The gamma-tubulin ring complex (γ-TuRC) is the principal microtubule nucleation template in vertebrates. Microtubules are formed de novo in a process termed nucleation, which is spatially and temporally highly controlled by γ-tubulin complexes, composed of γ-tubulin1 and associated γ-tubulin-complex proteins (GCP). In most eukaryotes, microtubules are templated from a preassembled γ-tubulin ring complex (γ-TuRC) that determines the position and direction of microtubule growth. Here, we used cryo-EM to identify and characterize γ-TuRC assembly intermediates after recombinant expression of the complex, which allowed us to delineate a comprehensive stepwise assembly pathway from a stable 6-spoked core to the mature 14-spoked γ-TuRC, identifying successive stabilization and conformational locking of γ-TuSC units as central principles in the assembly process.

The almost constant ratio between γ-TuSC(13,14)-containing and -lacking intermediates for each assembly step argues for repeated association and dissociation of γ-TuSC(13,14) in an equilibrium reaction. Stable incorporation of the γ-TuSC(13,14) unit, which is likely to repeatedly associate and dissociate over the assembly process, is a two-step process. Collectively, the observed intermediate steps can be arranged into a pathway for modular assembly of the γ-TuRC, in which the 6-spoke intermediate is expanded by successive recruitment of γ-TuSC units on the GCP2(7)-facing side while the γ-TuSC(13,14) unit repeatedly associates and dissociates until it is stabilized in the final step of complex assembly.

>[8x]MPREIITLQLGQCGNQIGFEFWKQLCAEHGISPEGIVEEFATEGTDRKDVFFYQADDEHYIPRAVLLDLEPRVIHSILNSPYAKLYNPENIYLSEHGGGAGNNWASGFSQGEKIHEDIFDIIDREADGSDSLEGFVLCHSIAGGTGSGLGSYLLERLNDRYPKKLVQTYSVFPNQDEMSDVVVQPYNSLLTLKRLTQNADCVVVLDNTALNRIATDRLHIQNPSFSQINQLVSTIMSASTTTLRYPGYMNNDLIGLIASLIPTPRLHFLMTGYTPLTTDQSVASVRKTTVLDVMRRLLQPKNVMVSTGRDRQTNHCYIAILNIIQGEVDPTQVHKSLQRIRERKLANFIPWGPASIQVALSRKSPYLPSAHRVSGLMMANHTSISSLFERTCRQYDKLRKREAFLEQFRKEDMFKDNFDEMDTSREIVQQLIDEYHAATRPDYISWGTQEQ;>MSEFRIHHDVNELLSLLRVHGGDGAEVYIDLLQKNRTPYVTTTVSAHSAKVKIAEFSRTPEDFLKKYDELKSKNTRNLDPLVYLLSKLTEDKETLQYLQQNAKERAELAAAAVGSSTTSINVPAAASKISMQELEELRKQLGSVATGSTLQQSLELKRKMLRDKQNKKNSGQHLPIFPAWVYERPALIGDFLIGAGISTDTALPIGTLPLASQESAVVEDLLYVLVGVDGRYVSAQPLAGRQSRTFLVDPNLDLSIRELVHRILPVAASYSAVTRFIEEKSSFEYGQVNHALAAAMRTLVKEHLILVSQLEQLHRQGLLSLQKLWFYIQPAMRTMDILASLATSVDKGECLGGSTLSLLHDRSFSYTGDSQAQELCLYLTKAASAPYFEVLEKWIYRGIIHDPYSEFMVEEHELRKERIQEDYNDKYWDQRYTIVQQQIPSFLQKMADKILSTGKYLNVVRECGHDVTCPVAKEIIYTLKERAYVEQIEKAFNYASKVLLDFLMEEKELVAHLRSIKRYFLMDQGDFFVHFMDLAEEELRKPVEDITPPRLEALLELALRMSTANTDPFKDDLKIDLMPHDLITQLLRVLAIETKQEKAMAHADPTELALSGLEAFSFDYIVKWPLSLIINRKALTRYQMLFRHMFYCKHVERQLCSVWISNKTAKQHSLHSAQWFAGAFTLRQRMLNFVQNIQYYMMFEVMEPTWHILEKNLKSASNIDDVLGHHTGFLDTCLKDCMLTNPELLKVFSKLMSVCVMFTNCMQKFTQSMKLDGELGGQTLEHSTVLGLPAGAEERARKELARKHLAEHADTVQLVSGFEATINKFDKNFSAHLLDLLARLSIYSTSDCEHGMASVISRLDFNGFYTERLERLSAERSQKATPQVPVLRGPPAPAPRVAVTAQ[2x];>MATPDQKSPNVLLQNLCCRILGRSEADVAQQFQYAVRVIGSNFAPTVERDEFLVAEKIKKELIRQRREADAALFSELHRKLHSQGVLKNKWSILYLLLSLSEDPRRQPSKVSSYATLFAQALPRDAHSTPYYYARPQTLPLSYQDRSAQSAQSSGSVGSSGISSIGLCALSGPAPAPQSLLPGQSNQAPGVGDCLRQQLGSRLAWTLTANQPSSQATTSKGVPSAVSRNMTRSRREGDTGGTMEITEAALVRDILYVFQGIDGKNIKMNNTENCYKVEGKANLSRSLRDTAVRLSELGWLHNKIRRYTDQRSLDRSFGLVGQSFCAALHQELREYYRLLSVLHSQLQLEDDQGVNLGLESSLTLRRLLVWTYDPKIRLKTLAALVDHCQGRKGGELASAVHAYTKTGDPYMRSLVQHILSLVSHPVLSFLYRWIYDGELEDTYHEFFVASDPTVKTDRLWHDKYTLRKSMIPSFMTMDQSRKVLLIGKSINFLHQVCHDQTPTTKMIAVTKSAESPQDAADLFTDLENAFQGKIDAAYFETSKYLLDVLNKKYSLLDHMQAMRRYLLLGQGDFIRHLMDLLKPELVRPATTLYQHNLTGILETAVRATNAQFDSPEILRRLDVRLLEVSPGDTGWDVFSLDYHVDGPIATVFTRECMSHYLRVFNFLWRAKRMEYILTDIRKGHMCNAKLLRNMPEFSGVLHQCHILASEMVHFIHQMQYYITFEVLECSWDELWNKVQQAQDLDHIIAAHEVFLDTIISRCLLDSDSRALLNQLRAVFDQIIELQNAQDAIYRAALEELQRRLQFEEKKKQREIEGQWGVTAAEEEEENKRIGEFKESIPKMCSQLRILTHFYQGIVQQFLVLLTTSSDESLRFLSFRLDFNEHYKAREPRLRVSLGTRGRRSSHT[4x];>MIHELLLALSGYPGSIFTWNKRSGLQVSQDFPFLHPSETSVLNRLCRLGTDYIRFTEFIEQYTGHVQQQDHHPSQQGQGGLHGIYLRAFCTGLDSVLQPYRQALLDLEQEFLGDPHLSISHVNYFLDQFQLLFPSVMVVVEQIKSQKIHGCQILETVYKHSCGGLPPVRSALEKILAVCHGVMYKQLSAWMLHGLLLDQHEEFFIKQGPSSGNVSAQPEEDEEDLGIGGLTGKQLRELQDLRLIEEENMLAPSLKQFSLRVEILPSYIPVRVAEKILFVGESVQMFENQNVNLTRKGSILKNQEDTFAAELHRLKQQPLFSLVDFEQVVDRIRSTVAEHLWKLMVEESDLLGQLKIIKDFYLLGRGELFQAFIDTAQHMLKTPPTAVTEHDVNVAFQQSAHKVLLDDDNLLPLLHLTIEYHGKEHKADATQAREGPSRETSPREAPASGWAALGLSYKVQWPLHILFTPAVLEKYNVVFKYLLSVRRVQAELQHCWALQMQRKHLKSNQTDAIKWRLRNHMAFLVDNLQYYLQVDVLESQFSQLLHQINSTRDFESIRLAHDHFLSNLLAQSFILLKPVFHCLNEILDLCHSFCSLVSQNLGPLDERGAAQLSILVKGFSRQSSLLFKILSSVRNHQINSDLAQLLLRLDYNKYYTQAGGTLGSFGM[2x];>[2x]MARHGPPWSRLDAQQERDVRELVRGVAGLQDEADPNFQLALNFAWSNFRFHRFLDVNSHKIEKTIEGIYEKFVIHSDLSKAASWKRLTEEFLNAPLPSIKEIKTDAHYSILSLLLCLSDSPSNSSYVETPRNKEVEKKDDFDWGKYLMEDEEMDIGPYMDTPNWSEESEEENDQQPLSREDSGIQVDRTPLEEQDQNRKLDPCISWKDEPDDRSWLEHHVVHQYWTARPSQFPHSLHLHSNLAAVWDQHLYSSDPLYVPDDRVLVTETQVIRETLWLLSGVKKLFIFQLIDGKVTVRNNIIVTHLTHSCLRSVLEQIAAYGQVVFRLQEFIDEVMGHSSESMLPGSGSVPKKSTEAPFRTYQAFMWALYKYFISFKEELAEIEKCIINNDTTITLAIVVDKLAPRLSQLKVLHKVFSTGVAEVPPDTRNVVRASHLLNTLYKAILEYDNVGEASEQTVSLLFSLWVETVRPYLQTVDEWIVHGHLWDGAREFIIQRNKNVPVNHRDFWYATYTLYSVSEKTENEEKMSDNASASSGSDQGPSSRQHTMVSFLKPVLKQIIMAGKSMQLLKNLQCAESTTCQAGARDAERKSLYTLFLESVQSRLRHGEDSTPQVLTEQQATKENLMKMQSIAESHLELDDVHDPLLAINFARMYLEQSDFHEKFAGGDVCVDRSSESVTCQTFELTLRSCLYPHIDKQYLDCCGNLMQTLKKDYRLVEYLQAMRNFFLMEGGDTMYDFYTSIFDKIREKETWQNVSFLNVQLQEAVGQRYPEDSSRLSISFENVDTAKKKLPVHILDGLTLSYKVPWPVDIVISLECQKIYNQVFLLLLQIKWAKYSLDVLLFGELVSTAEKPRLKEGLIHEQDTVAQFGPQKEPVRQQIHRMFLLRVKLMHFVNSLHNYIMTRILHSTGLEFQHQVEEAKDLDQLIKIHYRYLSTIHDRCLLREKVSFVKEAIMKVLNLALMFADGWQAGLGTWRMESIEKMESDFKNCHMFLVTILNKAVCRGSFPHLESLALSLMAGMEQS;> MASITQLFDDLCEALLPAAKTHLGQRSVNRKRAKRSLKKVAYNALFTNLFQDETQQLQPDMSKLPARNKILMLSFDLRVGGLGPKADRLEELVEELEAAPCCPLLEVGSVLDLLVQLAGSGPPQVLPRKRDYFLNNKHVGRNVPYSGYDCDDLSVFEMDVQSLISREECLCHSMIQETLQVMEAAPGTGLPTVGLFSFGDPCGDRFERDTRVSLFGALVHSRTYDMDVRLGLPPVPDNADLSGLAIKVPPSVDQWEDEGFQSASNLTPDSQSEPSVTPDVDLWEAALTYEASKRRCWERVGCPPGHREEPYLTEAGRDAFDKFCRLHQGELQLLAGGVLQAPQPVLVKECELVKDVLNVLIGVVSATFSLCQPAQAFVVKRGVHVSGASPESISSLLSEVAEYGTCYTRLSHFSLQPVLDSLYSKGLVFQAFTSGLRRYLQYYRACVLSTPPTLSLLTIGFLFKKLGRQLRYLAELCGVGAVLPGTCGGGPRAAFPTGVKLLSYLYQEALHNCSNEHYPVLLSLLKTSCEPYTRFIHDWVYSGVFRDAYGEFMIQVNHEYLSFRDKLYWTHGYVLISKEVEDCVPVFLKHIAHDIYVCGKTINLLKLCCPRHYLCWSDVPVPRISVIFSLEELKEIEKDCAVYVGRMERVARHSSVSKEEKELRMEIAKQELIAHAREAASRVLSALSDRQMSERMALDARKREQFQRLKEQFVKDQERRQAARQEELDDDFSYARELRDRERRLKSLEEELERKARQALVDHYSKLSAEAARREQKALWRIQRHRLESARLRFLLEDEKHIQEMLKAVSEAHQPQEPPDVLLSVHPQVTSPGPEHPEGGQGCDSGSAEQHSPAWDGWNRPGLLTPQPLKPLAVGAGGRGLQQAEGARPFSDSLSIGDFLPVGPGAEPSVQTGMVPLLEVALQTINLDLPPSAPGEAPAAASTQPSRPQEYDFSTVLRPAVATSPAPGPLQAAECSLGSSGLQLWEDSCGKMDACGSASRETLLPSHPPRRAALEEGSSQPTERLFGQVSGGGLPTGDYASEIAPTRPRWNTHGHVSDASIRVGENVSDVAPTQPRWNTHGHVSNASISLGESVSDVAPTRPRWNIHGHVSNASIRVGENVSDVAPTRPRWNTHGHVSNASIRVGENVSDVAPTRPRWNTHGHVSDASISLGESVSDMAPARPRWNTHGHVSDASISLGESVSDMAPTRPRWNTHGHVSDTSIRVGENVSDVAPIRSRCNTHGHVSDASISLGEPVSDVVSTRPRWNTHVPIPPPHMVLGALSPEAEPNTPRPQQSPPGHTSQSALSLGAQSTVLDCGPRLPVEVGPSLSSPSSGCGEGSISVGENVSDVAPTQPWWPNTPGDSVSEELGPGRSGDTEDLSPNWPLNSQEDTAAQSSPGRGEEAEASAAEAQGGEQAYLAGLAGQYHLERYPDSYESMSEPPIAHLLRPVLPRAFAFPVDPQVQSAADETAVQLSELLTLPVLMKRSITAPLAAHISLVNKAAVDYFFVELHLEAHYEALRHFLLMEDGEFAQSLSDLLFEKLGAGQTPGELLNPLVLNSVLSKALQCSLHGDTPHASNLSLALKYLPEVFAPNAPDVLSCLELRYKVDWPLNIVITEGCVSKYSGVFSFLLQLKLMMWALKDVCFHLKRTALLSHMAGSVQFRQLQLFKHEMQHFVKVIQGYIANQILHVTWCEFRARLATVGDLEEIQRAHAEYLHKAVFRGLLTEKAAPVMNVIHSIFSLVLKFRSQLISQAWGPPGGPRGAEHPNFALMQQSYNTFKYYSHFLFKVVTKLVNRGYQPHLEDFLLRINFNNYYQDA;>MASSSGAGAAAAAAAANLNAVRETMDVLLEISRILNTGLDMETLSICVRLCEQGINPEALSSVIKELRKATEALKAAENMTS[3x]> GSHMFC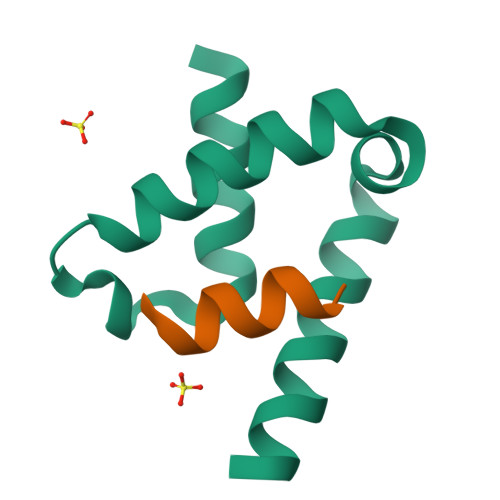EKYKQTKEQALTFFQEHPQYMRSKEDEEQLMTEFKKVLLEPGSKNLSIYQTLLAAHERLQAL;> DDKLQKWVRVYLDRGQ Jasmonates are phytohormones that are pivotal in mediating plant responses to various biotic and abiotic stresses and regulating plant growth. The first crystal structure of OPR3 from tomato (SlOPR3) showed that the enzyme crystallized as a self-inhibitory dimer in which the L6 loop, a critical loop involved in substrate recognition and coenzyme binding, from each protomer intrudes into the active site cavity of the other protomer. Based on these observations, it was postulated that the formation of the self-inhibitory homodimer represents a mechanism for regulating OPR3 activity and, thereby, jasmonic acid biosynthesis.

Variant Y364P was produced to test whether residue Y364 is required for homodimerization, as proposed previously. Proline was chosen because other well-studied ene-reductases, such as morphinone reductase, contain a proline at the corresponding position to Y364. Like the other variants, the monomeric form of Y364P is almost identical to the wild-type structure (RMSDCα = 0.21 Å) and misses nearly the entire loop L6 due to disorder. The sulfate binding site is identical to that in the wild-type homodimer, except for the absence of Y364. At the highest tested concentration (20 mg/ml), all samples, except for R283D, which was not completely soluble at this concentration, exhibited a hydrodynamic diameter of around 10 nm, agreeing well with the calculated values of 9.18–9.54 nm for the respective dimer. Interestingly, variant Y364P, which, because of the lack of Y364, was not expected to dimerize readily, showed a clear tendency for dimerization with increasing concentration. All enzymes (wild type and three variants) could be crystallized in their monomeric and dimeric forms, even variant Y364P, which lacks the putative phosphorylation target Y364.

> HHHHHHMASSAQDGNNPLFSPYKMGKFNLSHRVVLAPMTRCRALNNIPQAALGEYYEQRATAGGFLITEGTMISPTSAGFPHVPGIFTKEQVREWKKIVDVVHAKGAVIFCQLWHVGRASHEVYQPAGAAPISSTEKPISNRWRILMPDGTHGIYPKPRAIGTYEISQVVEDYRRSALNAIEAGFDGIEIHGAHGYLIDQFLKDGINDRTDEYGGSLANRCKFITQVVQAVVSAIGADRVGVRVSPAIDHLDAMDSNPLSLGLAVVERLNKIQLHSGSKLAYLHVTQPRYVAYGQTEAGRLGSEEEEARLMRTLRNAYQGTFICSGGYTRELGIEAVAQGDADLVSYGRLFISNPDLVMRIKLNAPLNKPNRKTFYTQDPVVGYTDYPFLQGNGSNGPLSRL>[2x]AHHHHHHSSGLEVLFQGPPEGAALTEKTDIFESGRNGNPNKDGIKSYRIPALLKTDKGTLIAGADERRLHSSDWGDIGMVIRRSEDNGKTWGDRVTITNLRDNPKASDPSIGSPVNIDMVLVQDPETKRIFSIYDMFPEGKGIFGMSSQKEEAYKKIDGKTYQILYREGEKGAYTIRENGTVYTPDGKATDYRVVVDPVKPAYSDKGDLYKGDQLLGNIYFTTNKTSPFRIA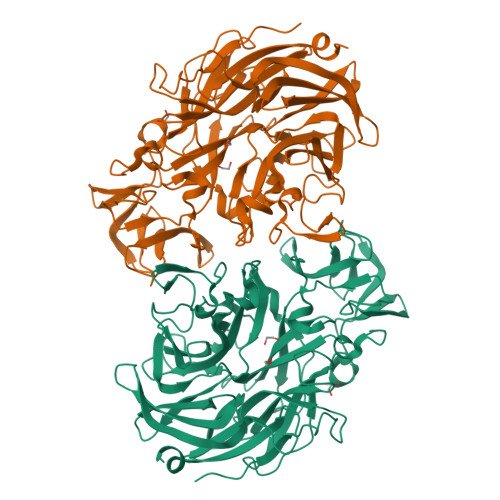KDSYLWMSYSDDDGKTWSAPQDITPMVKADWMKFLGVGPGTGIVLRNGPHKGRILIPVYTTNNVSHLDGSQSSRVIYSDDHGKTWHAGEAVNDNRQVDGQKIHSSTMNNRRAQNTESTVVQLNNGDVKLFMRGLTGDLQVATSKDGGVTWEKDIKRYPQVKDVYVQMSAIHTMHEGKEYIILSNAGGPKRENGMVHLARVEENGELTWLKHNPIQKGEFAYNSLQELGNGEYGILYEHTEKGQNAYTLSFRKFNWEFLSKN octyl 2-O-(6-deoxy-alpha-L-galactopyranosyl)-beta-D-galactopyranoside 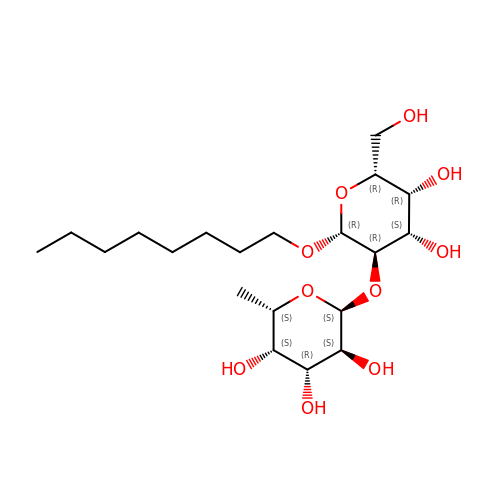| C20 H38 O10 | GTTDTLMUWQMDNA-ARNYJBIMSA-N>[4x]MGHHHHHHHHHHSSGHIEGRHMMATNLRGVMAALLTPFDQQQALDKASLRRLVQFNIQQGIDGLYVGGSTGEAFVQSLSERAQVLEIVAEEAKGKIKLIAHVGCVSTAESQQLAASAKRHGFDAVSAVTPFYYPFSLEEHCD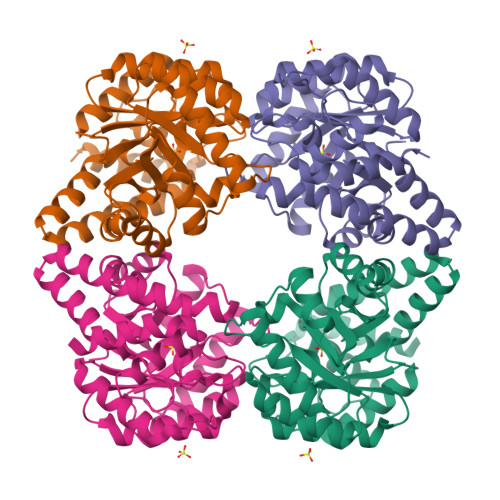HYRAIIDSADGLPMVVYNIPALSGVKLTLGQIYTLVTLPGVGALKQTSGDLYQMEQIRREHPDLVLYNGYDEIFASGLLAGADGGIGSTYNIMGWRYQGIVKALKEGDIQTAQKLQTECNKVIDLLIKTGIFRGLKTVLHYMDVISVPLCRKPFGPVDEKCLPELKALAQQLMQERG> IDPFTMGVITSESEYVSSLSAEKLYRGIVEDGNIIYPKALPRFIEKAETLEGDGGPGTIKKLTFVGDFGSTKQHIDMVDRENC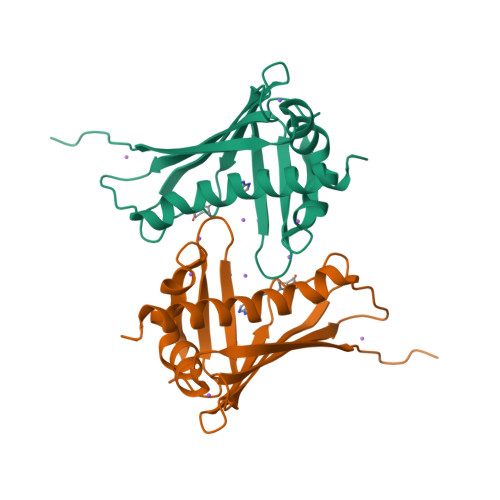AYTYSVYEGIALSDQPLEKIVFEFKLVPTPEEGCIVKSTTKYYTKGDDIELSKDYLEAGIERFEGFTKAVESFLLANPDYNKDSN> MYFQIRGIILWPRNKNFKPHTIRFELGKVNVISGASRTGKSAVIPIIDYCLGANTCSIPVKTIRKYCEWFGIVVATEQGEKLLARKEPGNQRSTTDMFVLEAENITSIPIRLEKNTNVIAVKRMLDDLANLSNLDFSGGDENSGFDGRPAFRDLAAFTFQPQNVVANPDVLFFKTNTYEHREKLRKIFPYVLGAITSELMAKQFELNRIRLFLRRKER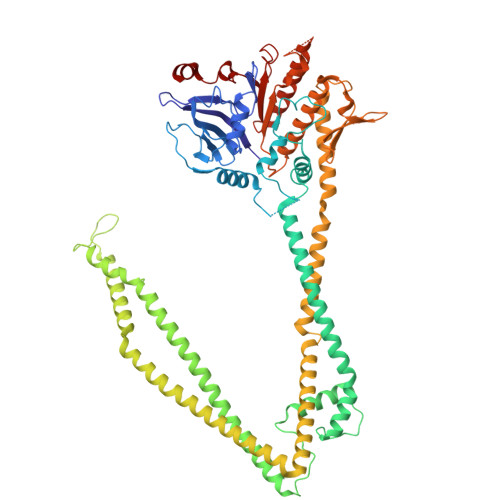ELKDAQDVSAQWLADLKSKYSEAQELGLVPKPQEQLSRKQMISQLEEVISRTDLTLKVTVSTISDALSELNTLESEERLVSRELTTMRHRLEEMNRLRVGMHQYENALLMQRDRLKISGWLLSNTNDESDCPMCGSHTDSAKQKLQALVQRLSDVEAAVGADAHKEVPAAFDRELQRVTTEVANATERLRAIQSRKRTLTSRSKEAREQQFSTRRAERFIGNVESALELHRKLGSDSELVEEVRKLKEMVQTLEKELREKDVELRKNQALRVINAQAGNILQGLDVEDPSAPISLEINDLTIKVLGDERDDYLSEIGSGSNWLSYHLAILLSLHQFYLSQKNNPVPSFLILDQPSQVYFPKTTQLPNIANEDEPKLRDEDVEAVRRAFKAMGNVVIKEKGKLQLIVLDHAPREVWGEIDGVVGLPEWRDGIKLVPMEWLTGV N-3-OXO-DODECANOYL-L-HOMOSERINE 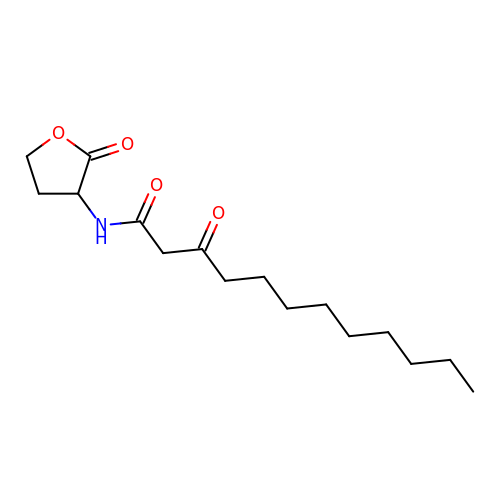LACTONE | C16 H27 N O4 | PHSRRHGYXQCRPU-AWEZNQCLSA-N>MKHHHHHHHHGGLVPRGSHGGSSRSRLIAQAVGPATVLAMGKAVPANVFEQATYPDFFFNITNSNDKPALKAKFQRICDKSGIKKRHFYLDQKILESNPAMCTYMETSLNCRQEIAVAQVPKLAKEASMNAIKEWGRPKSEITHIVMATTSGVNMPGAELATAKLLGLRPNVRRVMMYQQGCFAGATVLRVAKDLAENNAGARVLAICSEVTAVTFRAPSETHIDGLVGSALFGDGAAAVIVGSDPRPGIERPIYEMHWAGEMVLPESDGAIDGHLTEAGLVFHLLKDVPGLITKNIGGFLKDTKNLVGASSWNELFWAVHPG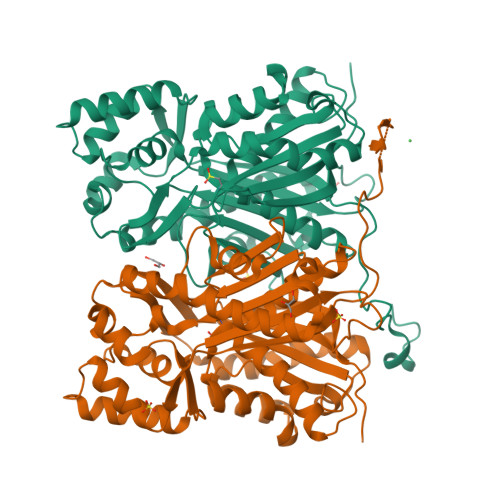GPAILDQVEAKLELEKGKFQASRDILSDYGNMSSASVLFVLDRVRERSLESNKSTFGEGSEWGFLIGFGPGLTVETLLLRALPLQQAERV[2x]>MKSRIIVRTSFDAAHAVKVGDHWEDVHGHTFFLEVAIEGEIKNGYVMDFLELRKIVEEITKELDHRNLNNIFENPTTENIALWIGERIRDKLPPYVKLKRVV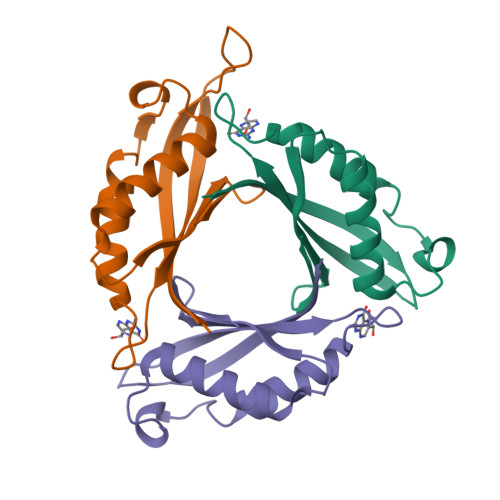LWEGKDNGVELEW[6x]Here, we report the de novo design of a TIM barrel with ovoid (twofold) symmetry, drawing inspiration from natural beta and TIM barrels with ovoid curvature. To this end, we report the computational design and experimental validation of a de novo ovoid TIMB protein, with a completely novel syntax and sequence. The designed protein exhibits an elongated β barrel architecture with loops which are not structurally involved and a more developed hydrophobic core. In accordance with our design goals, the protein folds solubly and is highly stable.

In order to assess whether the proteins fold as designed, and especially whether the ovoid β barrel curvature is maintained, we determined the 3D structure of the OT3 design by X-ray crystallography using molecular replacement with the design model. The experimental structure aligns with high accuracy to the design model, with an overall Cα RMSD of 1.59 Å. In particular, the β barrel showed excellent fidelity, exhibiting just 0.74 Å RMSD over α and β carbon atoms and mirroring closely the ovoid curvature specified in the computational design. Side chain packing in the hydrophobic regions also closely followed the designed rotamers. Especially, the close packing around A93 and A207 suggests that the placement of sterically small residues at the ovoid barrel minor face was a successful strategy. The redesigned β-α loops are free of any critical hydrogen bonding or structural interactions as in the original sTIM11, enabling their redesign and diversification. To assess the quality of the twofold symmetry design, we aligned the first repeat subunit to the second and found close agreement (0.74 Å Cα RMSD), indicating that the designed twofold symmetry is self-consistent and viable. Deviations between the design model and crystal structure can be largely explained by shifting of the helices and loops and may point to potential targets for future redesign. We noticed two main points of deviation: disagreement between the fourth and eighth helices (α4 and α8, which are symmetry mates) and the design model and disagreement between the seventh helix (α7) and the design model (these can be observed in Figure 2d). The total hydrophobic contacts and total buried area across all clusters are increased significantly in OT3 (174 contacts; 7864.8 Å2) compared to sTIM11 (81 contacts; 4067.8 Å2). However, visual inspection reveals that previous flaws with sTIM11 are eliminated in OT3, such as a cavity in the central β barrel and gaps between each of the hydrophobic clusters.

> MHHHHHHENLYFQSDAICIYLDESATWKDMKKAMEILYKLGVKKIVVLFKYDEKLIKVAAKVLHDLGAEEAIIILIFDIDDEDEFKKQVKKALELMKKLGVDHRIIALRMTDEEKFKKLAKIAAELGADAICIYLDESATWKDMKKAMEILYKLGVKKIVVLFKYDEKLIKVAAKVLHDLGAEEAIIILIFDIDDEDEFKKQVKKALELMKKLGVDHRIIALRMTDEEKFKKLAKIAAELGA>MSQYSIQQSLGNASGVAVSPINADATLSTGVALNSSLWAGIGVFARGKPFTVLAVTESNYEDVLGEPLKPSSGSQFEPIRHVYEAIQQTSGYVVRAVPDDAKFPIIMFDESGEPAYSALPYGSEIELDSGEAFAIYVDDGDPCISPTRELTIETATADSAGNERFLLKLTQTTSLGVVTTLETHTVSLAEEAKDDMGRLCYLPTALEARSKYLRAVVNEELISTAKVTNKKSLAFTGGTNGDQSKISTAAYLRAVKVLNNAPYMYTAVLGLGCYDNAAITALGKICADRLIDGFFDVKPTLTYAEALPAVEDTGLLGTDYVSCSVYHYPFSCKDKWTQSRVVFGLSGVAYAAKARGVKKNSDVGGWHYSPAGEERAVIARASIQPLYPEDTPDEEAMVKGRLNKVSVGTSGQMIIDDALTCCTQDNYLHFQHVPSLMNAISRFFVQLARQMKHSPDGITAAGLTKGMTKLLDRFVASGALVAPRDPDADGTEPYVLKVTQAEFDKWEVVWACCPTGVARRIQGVPLLIK[12x]

The phage tail is a macromolecular machine responsible for specifically recognizing host bacteria, penetrating the cell membrane, and forming a channel for genome delivery. The conserved structural components include three main parts: a baseplate, a long inner tail tube, and a tail sheath that wraps around the tube. Phage P1, a temperate phage first discovered in 1951, transfers DNA into a wide range of gram-negative bacterial species by universal transduction and has been used to construct a fine structural genetic map of E. coli. During the tail-contraction, the tail sheath undergoes a massive conformational change and contracts to half and more of its original length, exposing the inner tail tube and providing the energy to drive the tail tube to eventually penetrate the target cell membrane.

Similarly, we resolved a partial contracted tail structure, including 15 sixfold sheath rings, at 3.9 Å, which also allowed us to build the atomic models for the tail sheath protein gp22. The tail terminator and tail tube structures did not resolve at high resolution, probably due to the different helical parameters between the sheath and the tail tube in the contracted tail, resulting in the problem of center-alignment. Tail-contraction causes the length of the tail sheath to decrease to 940 Å, and the width of the sheath to increase to 275 Å, and the pore diameter of each sheath ring to increase from 82 Å to 108 Å, resulting in the tail tube’s detachment from the sheath. Vertical compression of the sheath results in a smaller helical rise of 18 Å and a larger twist of 32°. The separation of the tail tube from the sheath provides the necessary conditions for the tail tube to penetrate the membrane. Structural comparison of the sheath protein gp22 in the extended and contracted states revealed that the dramatic conformational changes occur at the N-terminus and C-terminus. Specifically, the C-terminus of gp22 oscillates at a small angle, whereas the N-terminus oscillates upward by nearly 100°. Remarkably, the “handshake” and β-sheet augmentation mechanisms of the sheath–sheath interaction are still preserved in the contracted states. Our structures confirm that the N-terminus and C-terminus of the sheath act as a hinge, while the rest of the sheath acts as a rigid-body motion. The baseplate was not found in our contracted tail, suggesting that some degree of damage to the baseplate during sample preparation led to its detachment.>[4x]MRGSHHHHHH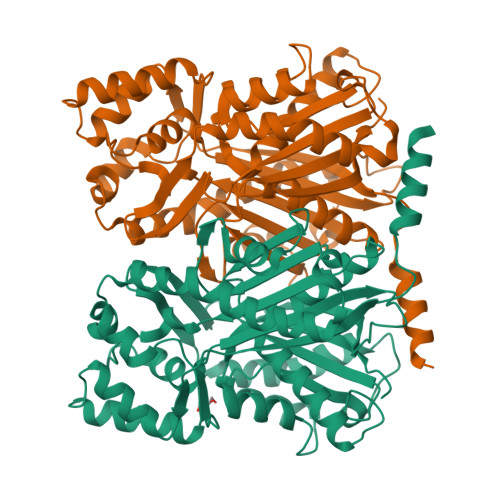GSMAKVKNFLNAKRSKGPASILAIGTANPPTCFNQSDYPDFYFRVTDCEHKTELKDKFKRICDRSAVKKRYLHVTEEVLKENPSMRSYNAPSLDARQALLIEQVPKLGKEAAAKAIKEWGQPLSKITHLVFSAMAGVDIPGADLRLMNLLGLEPSVKRLMIYSQGCFIGGAAIRCAKDFAENNAGARVLVVFSDIMNMYFHEPQEAHLDILVGQAVFGDGAAAVIVGADPEVSIERPLFHVVSSTQMSVPDTNKFIRAHVKEMGMELYLSKDVPATVGKNIEKLLVDAVSPFGISDWNSLFYSVHPGGRAILDQVELNLGLGKEKLRASRHVLSEYGNMGGSSVYFILDEIRKKSMQEAKPTTGDGLEWGVLFAIGPGLTVETVILLSVPIDSAC>[2x]MNTKYNKEFLLYLAGFVDGDGSIIAQIKPNQSHKFKHQLSLTFQVTEKTQRRWFLDKLVDEIGVGYVRDRGSVSDYILSEI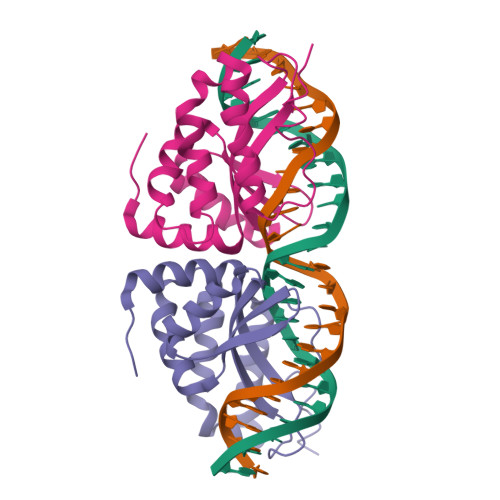KPLHNFLTQLQPFLKLKQKQANLVLKIIEQLPSAKESPDKFLEVCTWVDQIAALNDSKTRKTTSETVRAVLDSLSEKKKSSP>[2x]MKDWLFRIATCSIMTFSSLAAAQAEPLDVVATFSIIGDFAAKVGGDRIRLNVLVGPDSDTHVYEPRPADAIALAGADVVLTNGLEFEGFLTRLIAASGTDAAVATLTDGVETMEEPGGGGAHDPHAWQAVPNAKVYVQNIAAAFCAADAEGCAAYQANAARYIGELDALDTEIRAAIAALPQDRRTVVVAHNAFRYFEAAYGVHFLSPQGV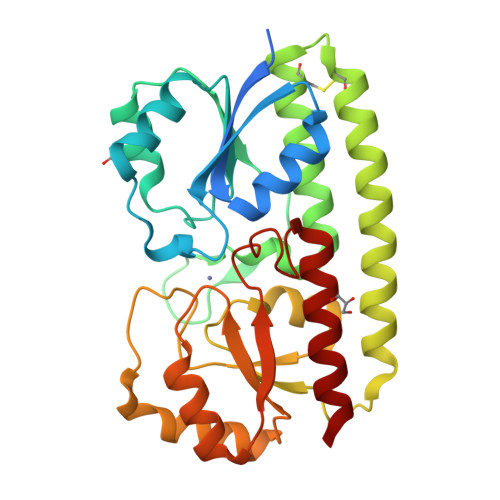STESEAAAADVAGLIREIRARNASAIFAENISDTRLLEQIAREAGLPLAGTLYSDALSGPDGPASNYIAMMRHNAGAIAAALAAR> GNELEKGNDGSGTVDPVNASTLVNVYSDKSGSEASLLVGDVLVKDSRTLTLNVPAACEKVYMKYNTVSGTEATKEFALSPVSRGVDQSTGFNFETNRLASVTLALPEDAVQPTNETDQGYLFYHNTGVVMFEDGWPIQLDSWYDEDFNDVVFEYDLKVTECHSQQMMETVGGKEELLLTLDVRAVGGIYPTVLGVVLDGLKSEYVDRITASLILKGGQGTMTDLAKEELSTKNIVKVENKNWNWSNDTRKEPRFAILTVDKAQAEGTVITLDGLTSLMDNNQDMFQVTQGKVREGLPML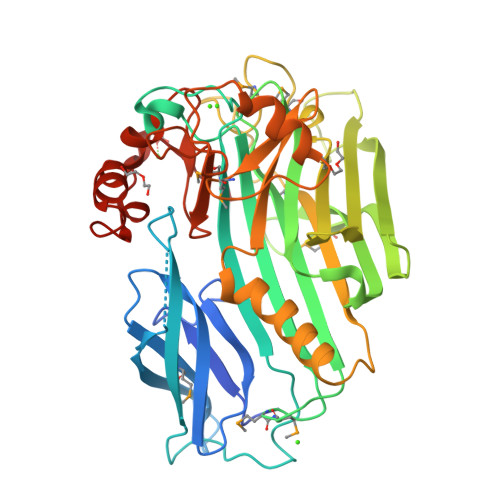RAEVRLIGKEGLTGAERDAQLAAFRELILDTNRQNFFIKVNGGKEIHMRGYAPTSAYKAEYEALVAGDTTLDANVYYSNTKGSTWGVKLPVGTRHAYERVPFREAYPDFTKWVDSKGVSNQKWYENFVDEKTIRYW> MKFTVGNGQNQHKGVNDGFSYEIWTNGGEGSMTLGSGATFKAEWNAAVNRGNFLARRGLDFGSQKKATDYDYIGLDYAATYKQTASASGNSRLCVYGWFQNRGLNGVPLVEYYIIEDWVDWVPDAQGKMVTIDGAQYKIFQMDHTGPTINGGSETFKQYFSVRQQKRTSGHIT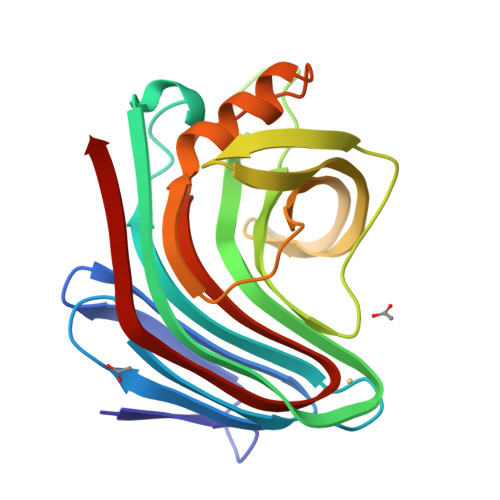VSDHFKEWAKQGWGIGNLYEVALNAEGWQSSGVADVTLLDVYTT>AIADVGTDRYAPYFAYAAAQPSDEVTTVRGLSNPLIKTAPVTLPFDLGQAVADNCLSLSGMGYYLGLGGCCPTCAAAEPRLGRSDRAALVLAYVQQLNSIYEYRVFLASVAARDPSERALEEVLAHPELFFAYYVLRDGGLRDVRVLFFEDPDAQGALMMYVVFPEKSVHVHHRVLDRLLGACAGHRIVAHVWQTMFVLVVRKKGDGRPADDVPAVSASDIYCKMRDISFDGELLLEYKRLYAAFEDFRPPRP[42x];>MSGTLVQRLKLILSGGNLRCSDGETACDPERPPTRCVFQVHGQDGSNDTFPLEYVLRLMRSWAHVPCDPYVRVQNTGVSVLFQGFFFRPADAPLAAITAEHNNVILASTHSTGMSLSALDDIKRAGGVDTRPLRAMMSVSCFVRMPRVQLSFRFMGPDDASQTQRLLDRAEMRQRSVSR[42x]

Although nucleo-cytoplasmic transport is typically mediated through nuclear pore complexes, herpesvirus capsids exit the nucleus via a unique vesicular pathway. Together, the conserved herpesvirus proteins pUL31 and pUL34 form the heterodimeric nuclear egress complex (NEC), which, in turn, mediates the formation of tight-fitting membrane vesicles around capsids at the inner nuclear membrane. In the nucleus of infected cells, pUL34 recruits pUL31 to the inner nuclear membrane to form the nuclear egress complex (NEC). Thus, the NEC represents self-sufficient machinery that can mediate inwardly directed vesicle formation.

To study the assembly of the heterodimeric complex into a hexagonal lattice, the former was fitted into the cryo-EM map derived from cells forming native NEC-coated vesicles. A lattice model was generated by global rotational search of the heterodimer and applying 6-fold symmetry; no further constraints were applied (for more details, see Experimental Procedures). The modeling resulted in the location of pUL34 most proximal to the membrane, thus validating the overall orientation of the fit. The long axis of the heterodimer is tilted by ∼70° relative to the membrane plane, i.e., being 20° off from a perpendicular orientation to the membrane. Our hexamer model indicates that pUL34 loop 88–93, as well as the pUL31 ZNF and loop 77–79, forms the intra-hexamer interface stabilized by hydrophobic interactions. To form a defined curved lattice that is key for successful budding as observed in situ (Hagen et al., 2015), the inter-hexamer interactions also have to be specific. These are established between hexamers at both trimer and dimer interfaces. Our model suggests that the hexamers’ trimeric interface is formed by pUL31 helix α5 and that the dimeric interface is formed by pUL34 loop 22–26, each interacting with their counterparts on the neighboring hexamer. Finally, the fit in lattice arrangement provides an indication where herpesvirus capsids as NEC cargo are likely to bind. The membrane-distal face of pUL31 is thereby suggested to form the inner coat of the cargo vesicles. Overall, the fit, based solely on a combined clash and protrusion score while not taking any mutation information as constraints, is consistent with previously reported data and results from our analyses presented here.>MLLERDLIQSVGFRNVREGGEITGFQFRVRMPSYRGMAASLIDGIGVRIPGLVDVGPDVPLWTLQGQQYTLAELWDGDGVRWPLEDAAIIFVPLPGGLPDGVHELSIELRLRMSYIPQEHQPSTYRVTKHVTLAPEASGAPFRYGVSLYSYMSDYGTVMDLETAMASIADLGATGIEILGEAHVPNYPNPSDEWVEQWFALLSTYGLEPTNMGSWIDTRLHSSGPNGRDMTVEEGAAALQRDLRLAKRLGFRFVRPKIGVVSSDLIPHPIWTEVVEASLPLAEELDVIICPEIHSPTPIKHEVVDDYIALIRRTGTKHFGLLLDTGIFQ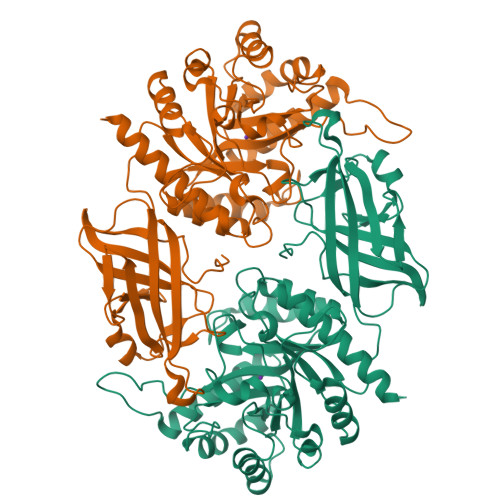DRPIPLKPGELPGQRPAFLDGIHVDPNDVFDVIENVVFIQAKFHDIDEELDDKQIPWEPVLKALKDAGYTGYLSSEYEGEREPWRSIEQVRRQHSLIRQIADRLAE[4x]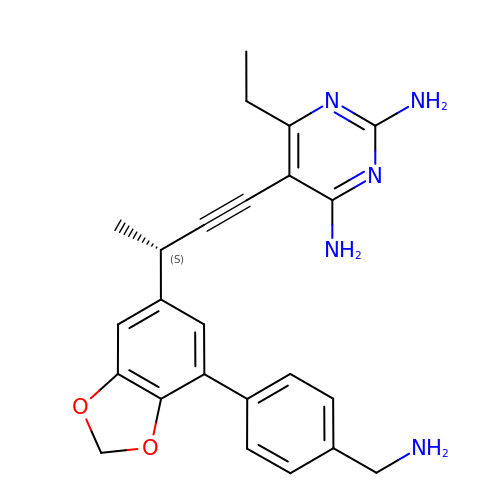5-[(3S)-3-{7-[4-(aminomethyl)phenyl]-2H-1,3-benzodioxol-5-yl}but-1-yn-1-yl]-6-ethylpyrimidine-2,4-diamine | C24 H25 N5 O2 | IIAMZXQFRCVQRC-CQSZACIVSA-N>[14x]HHHHHHE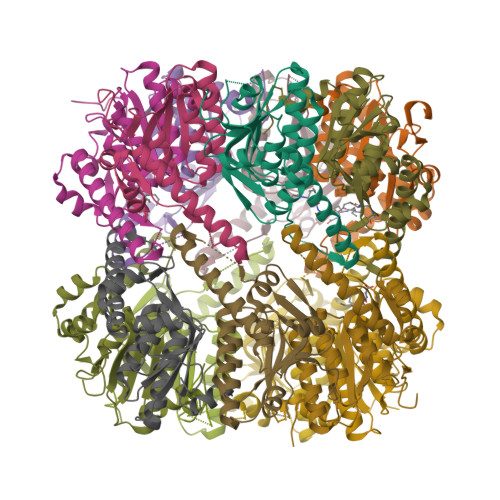NLYFQSNMSFDNYLVPTVIEQSGRGERAFDIYSRLLKERIVFLVGPVTDESANLVVAQLLFLESENPDKDIFFYINSPGGSVTAGMSIYDTMNFIKPDVSTLCLGQAASMGAFLLSAGEKGKRFALPNSRIMIHQPLISGGLGGQASDIEIHARELLKIKEKLNRLMAKHCDRDLADLERDTDRDNFMSAEEAKEYGLIDQILENRASLRL> DSTPDSLFAGLVGEYYGTNSQLNNISDFRALVDSKEADATFEAANISYGRGSSDVAKGTHLQEFLGSDASTL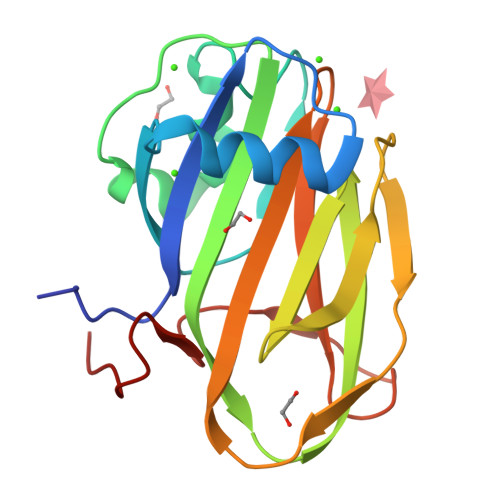STDPGDNTDGGIYLQGYVYLEAGTYNFKVTADDGYEITINGNPVATVDNNQSVYTVTHASFTISESGYQAIDMIWWDQGGDYVFQPTLSADGGSTYFVLDSAILSSTGETPYT>[6x]GPWFFGKIPRAKAEEMLSKQRHDGA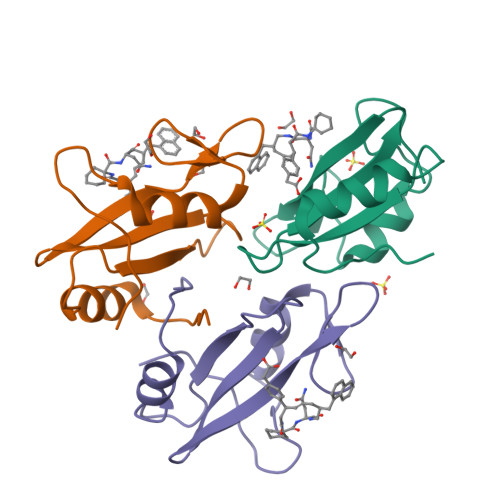FLIRESESAPGDFSLSVKFGNDVQHFKVLRDGAGKYFLWVVKFNSLNELVDYHRSTSVSRNQQIFLRDIE> SNAMGKVLSSSKEAAKLIHDGDTLIAGGFGLCGIPEQLILSIRDQGVKDLTVVSNNCGVDDWGLGLLLANKQIKKMIASYVGENKIFERQFLSGELEVELVPQGTLAERIRAGGAGIPGFYTATGVGTSIAEGKEHKTFGGRTYVLERGITGDVAIVKAWKADTMGNLIFRKTARNFNPIAAMAGKITIAEAEEIVEAGELDPDHIHTPGIYVQHVVLGASQEKRIE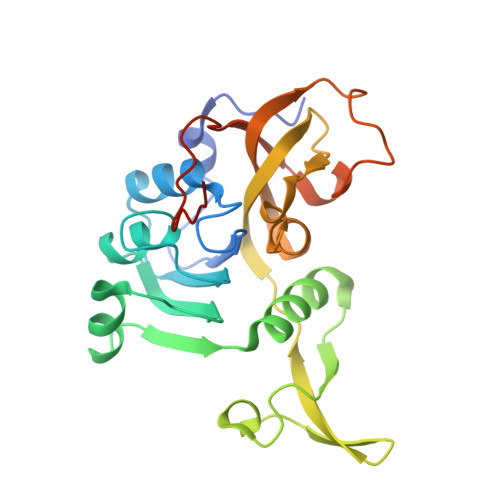KRTVQQASGKGEAK> GPEATLGSGNLRMAVMLPEGEDLNEWVAVNTVDFFNQINMLYGTITDFCTEESCPVMSAGPKYEYHWADGTNIKKPIKCSAPKYIDYLMTWVQDQLDDETLFPSKIGVP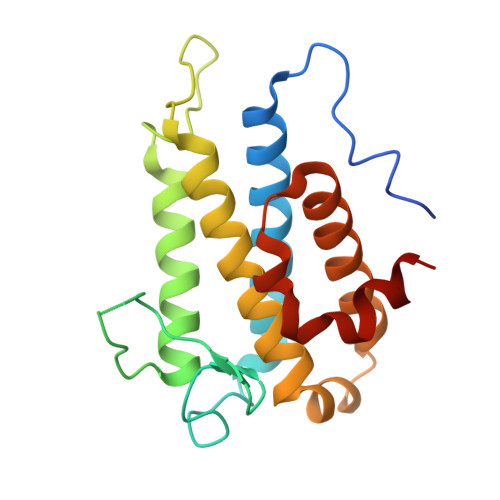FPKNFMSVAKTILKRLFRVYAHIYHQHFDPVIQLQEEAHLNTSFKHFIFFVQEFNLIDRRELAPLQELIEKLTSKDR7-[[(3R,4R)-3-(hydroxymethyl)-4-oxidanyl-pyrrolidin-1-ium-1-yl]methyl]-3,5-dihydropyrrolo[3,2-d]pyrimidin-4-one 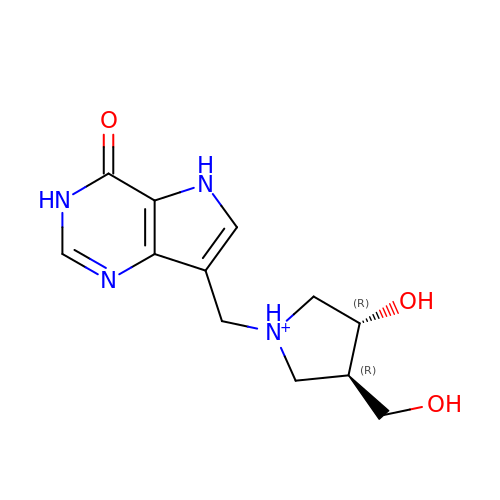| C12 H17 N4 O3 | AFNHHLILYQEHKK-BDAKNGLRSA-O>AGVAKFAKYPLTFGPSPISNLNRLSQHLGSKVNVYAKREDCNSGLAFGGNTLRKLEYIVPDIVEGDYTHLVSIGGRQSNQTRMVAALAAKLGKKCVLIQEDWVPIPEAEKDVYNRVGNIELSRIMGADVRVIEDGFDIGMRKSFANALQELEDAGHKPYPIPAGCSEHKYGGLGFVGFADEVINQEVELGIKFDKIVVCCVTGSTTAGILAGMAQYGRQDDVIAIDASFTSEKT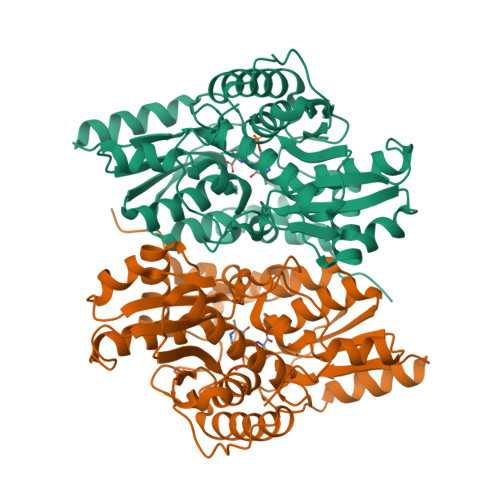KEQTLRIANNTAKLIGVEHEFKDFTLDTRFAYPCYGVPNEGTIEAIRTCAEQEGVLTDPVYEGKSMQGLIALIKEDYFKPGANVLYVHLGGAPALSAYSSFFPTKTA[4x]> GAKEYTNPKEGQLATTVSVKNNESTTPVRLLSKDTQGVEVTDTVSYSDLVGGKVYELTGTLMQIKADGSTEAIASASKEVTAETSGKGTWELTFAPQNLKAGEKYVVYEVAKSK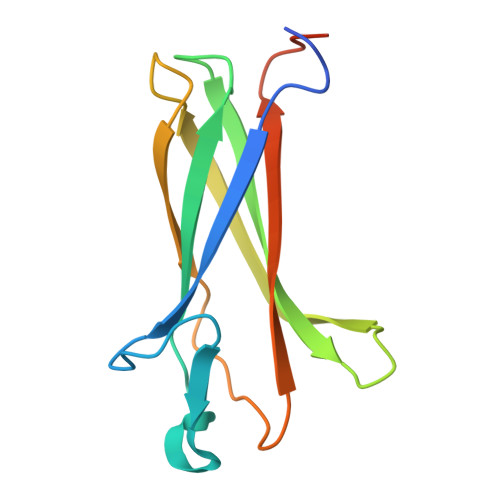ENLVDSNKDDESHG>[3x]MESSKTEQVTGATGITQSTVTAPLPEAVSSLSLAPTVNALDPWVYLNQTEVPGGTFTVSSATQPGSVLLELEISPELNLYTSHLFRMYAGWSGGFSLKLLVAGNAFSAGKLIAAIIPPNIEVPNSAYLLTGFPHEILDFRTADSMEIIAPDIKNIDYHFRGDKLGKLVVMVYSPLRSTSADFEIEIKLTSAPLPDFKFTMLVPPIQNNALPIWSIPQAPPYSMVNPRSPLTPVVELYINSSYATCNHQLGRYTIYQGAIGNSTFNPSGAWTATCTAEAGSVTGHPNWRYALLDLPDNPTFDPTLPPVPRGFCDWGSG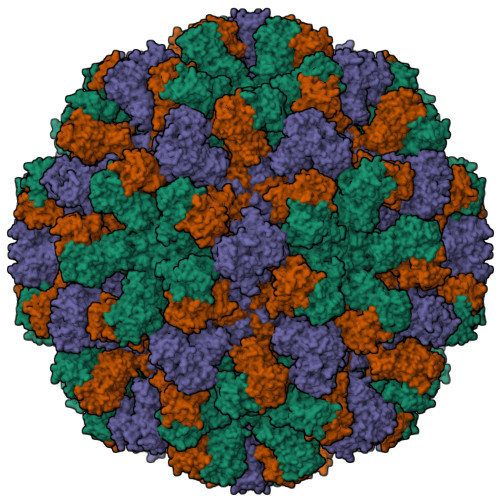VKSGNKQHLVCFTGKKVEGGFQDVDTHMWDYGDNETVGLDNTYQRTIYIKDPSLEKDAQYLVIPMGVSGAANDDTVQVAPNCYGSWDYAPTVAPPLGEQFVWFRSQLPASKTTTTSGVNSVPVNVNALMSPDLMCSAYASGFPLGKVALLDYVLFGGSVVRQFKLYPEGYMTANTTGSNTGFIIPADGYFRFNSWVSPSFMISSVVDLNLQTAVVFR>SNAMARLSQEIILNMAEKIIYEKGMEKTTLYDIASNLNVTHAALYKHYRNKEDLFQKLALRWLEETSREIFAWTQDAGQTPDDALHDWLWLLADTKKKRYKTDRKMFLLYTDYIEQNEELVKNHVAHLAQKAEEVSGRTNQGNAIITAFTYFHNPYFASRWEQAGY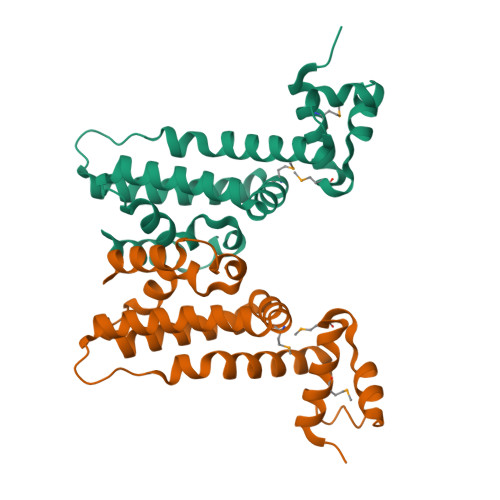VDLFEDVWQIVK[2x]>[2x]GSVYPKELTQVFEHYINNNLFDIDSLVKFIEELGYNLEDLATLCLAHLLGYKKLEEPLKREDFLSTWFMQGCSTISDMQECIKTLDVKLHEDLQYFTQIYNYAFNLILD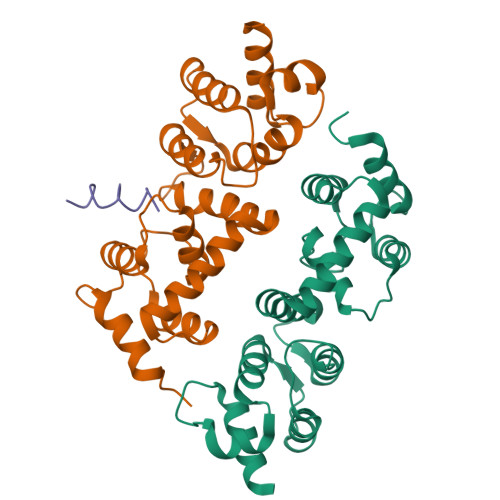PNRKDIDTDEGIQYWKLFFQPEYPVRMEPDLLEAWFRFLRDEGKTTISKDTWRMLLLFFKRYPTIQKIISDYDETAAWPFIIDEFYECLQDQQ;>XMLKLRQLQKKKQKENENSSSIQPN[2x]>[4x]GMQKLTRINDFNEVLNSRKSVKVFDENYKIPREEMDEIITKATKAPSSVNMQPWRIAVVQSDEMKEKVKESFGFNSRQLTTSSAMLIIFGDLQNYEKAEQIYGDAVEQQLM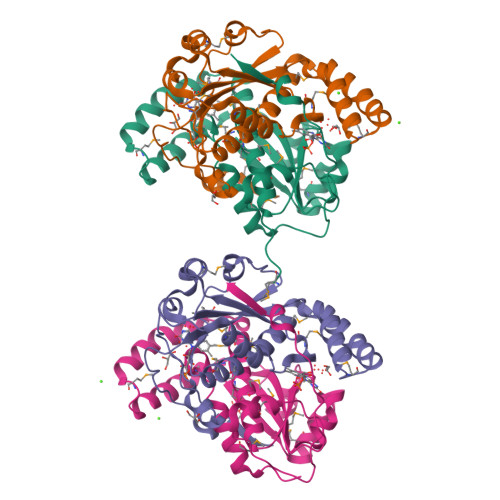TEDIKAQLLDWILPYYKNLSREGMKDIVNIDSSLMAMQLMLTAKAHGYDTNPIGGFDKENIADIIGYDSDRYVPVLAIAIGKKAQDAHDSVRLPIDDVREFL>[2x]GLVPRGSHMEVVVSFNDLSQPFFVAMRRELEDEAAKLGVKVQVLDAQNNSSKQISDLQAAAVQGAKVVIVAPTDSKALAGAADDLVEQGVAVISVDRNIAGGKTAVPHVGADNVAGGRAMADWVVKTYPAGARVVVITNDPGSSSSIERVKGVHDGLAAGGPAFKIVTEQTANSKRDQALTVTQNILTSMRDTPPDVILCLNDDMAMGALEAVRAAGLDSAKVKVIGFDAI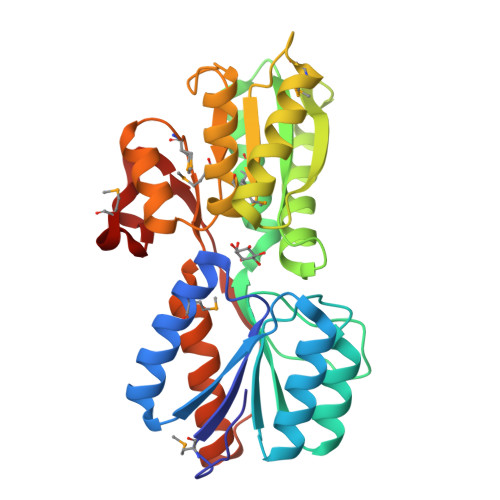PEALARIKAGEMVATVEQNPGLQIRTALRQAVDKIKSGAALKSVSLKPVLITSGNLTEASRIGEM> MQVNRLPFFTNHFFDTYLLISEDTPVGSSVTQLLARDMDNDPLVFGVSGEEASRFFAVEPDTGVVWLRQPLDRETKSEFTVEFSVSDHQGVITRKVNIQVGGVNDNAPTFHNQPYSVRIPENTPVGTPIFIVNATDPDLGAGGSVLYSFQPPSPFFAIDSARGIVTVIQELDYEVTQAYQLTVNATDQDKTRPLSTLANLAI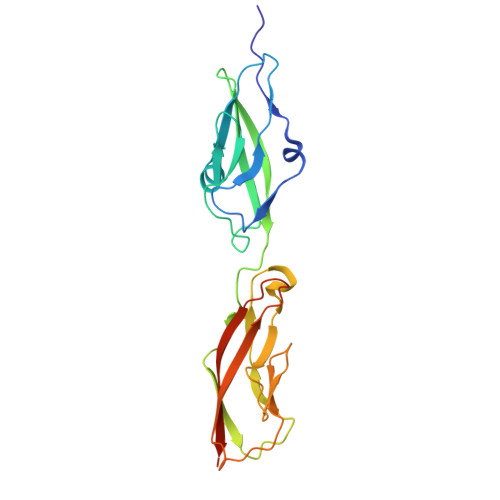IITDLEHHHHHH> SNAQIIFNVHPAPTRKIAVAKQNYRCAGCGIRTDPDYIKRLRYCEYLGKYFCQCCHENAQMAIPSRVLRKWDFSKYYVSNFSKDLLIKIWNDPLFNVQDINSALYRKVKLLNQVRLLRVQLCHMKNMFKTCRLAKELLDSFDTVPGHLTEDLHLYSLNDLTATRKGELGPRLAELTRAGATHVERCMLCQAKGFICEFCQNEDDIIFPFELHKCRTCEECKACYHKACFKSGSCPRCERLQARREALARQSLES;> SNATSRKKVLLKVIILGDSGVGKTSLMNQYVNKKFSNQYKATIGADFLTKEVMVDDRLVTMQIWDTAGLERFQSLGVAFYRGADCCVLVFDVTAPNTFKTLDSWRDEFLIQASPRDPENFPFVVLGNKIDLENRQVATKRAQAWCYSKNNIPYFETSAKE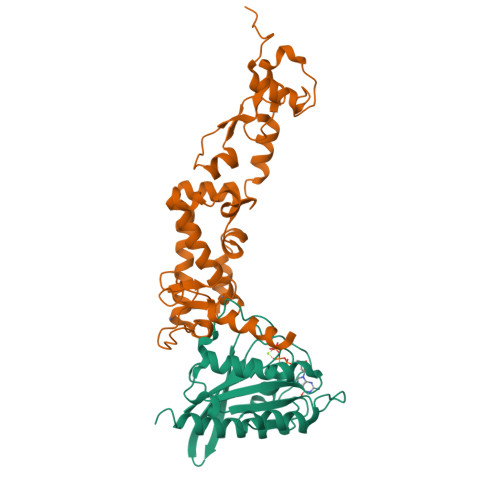AINVEQAFQTIARNALKQETEVEL> XAEKA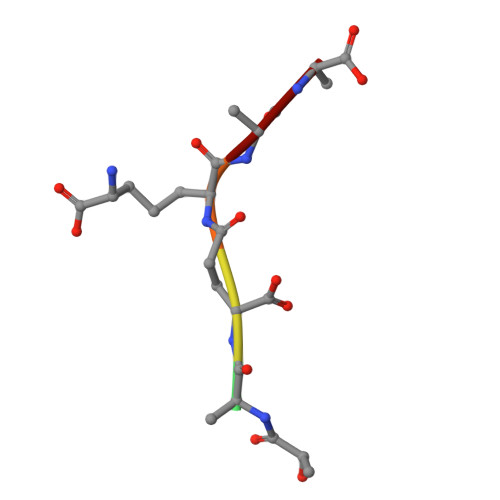A> GPHMSTSSANEDMPVEKILEAELAVEPKTETYVEANMGLNPSSPNDPVTNICQAADKQLFTLVEWAKRIPHFSELPLDDQVILLR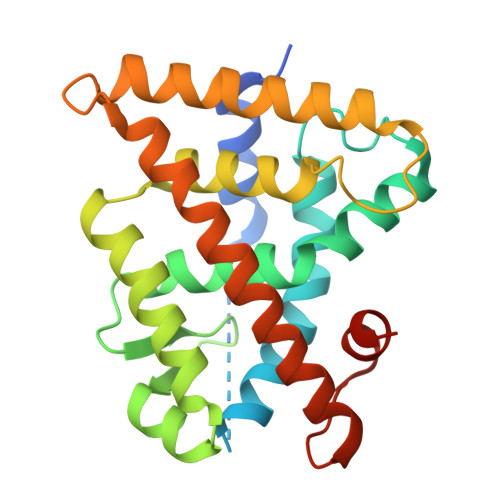AGWNELLAASASHRSIAVKDGILLTTGLHVHRNSAHSAGVGAIFDRVLTELVSKMRDMQMDKTELGCLRAIVLFNPDSKGLSNPAEVEALREKVYASLEAYCKHKYPEQPGRFAKLLLRLPALRSIGLKCLEHLFFFKLIGDTPIDTFLMEMLEAPHQAT> GCGCACUGGCGCUGCGCCUUCGGGCGCCAAUCGUAGCG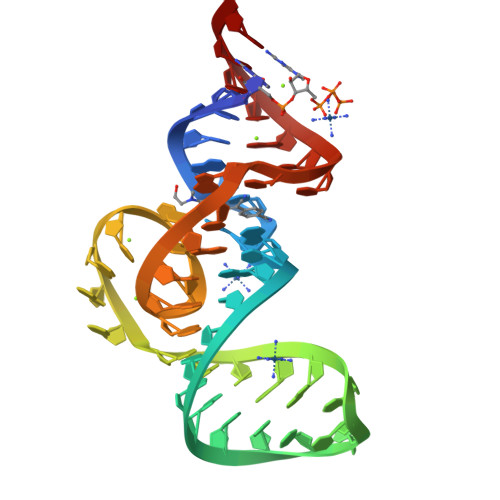UGUCGGCGCC> MKRQGKRPSKNLKARCSRKALHVNFKDMGWDDWIIAPLEYEAFHCEGLCEFPLRSHLEPTNHAVIQTLMNSMDPESTPPTCCV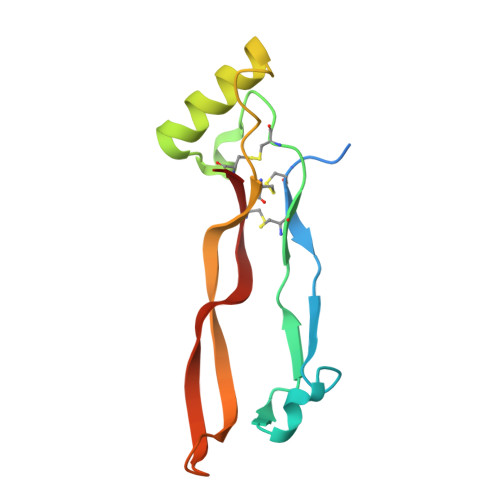PTRLSPISILFIDSANNVVKKDYEDMVVESCGCR1-[(5-chloro-1H-imidazo[4,5-b]pyridin-2-yl)methyl]-4-[(2-chloro-4-methoxyphenyl)methyl]-3-ethyl-1,3-dihydro-2H-imidazol-2-one 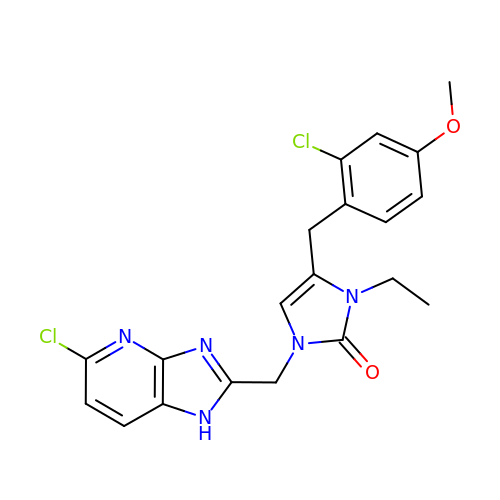| C20 H19 Cl2 N5 O2 | RDYREYRDYHMQKI-UHFFFAOYSA-N>[2x]MGHHHHHHHHHHSSGHIEGRHMMAERKGTAKVDFLKKIEKEIQQKWDTERVFEVNASNLEKQTSKGKYFVTFPYPYMNGRLHLGHTFSLSKCEFAVGYQRLKGKCCLFPFGLHCTGMPIKACADKLKREIELYGCPPDFPDEEEEEEETSVKTEDIIIKDKAKGKKSKAAAKAGSSKYQWGIMKSLGLSDEEIVKFSEAEHWLDYFPPLAIQDLKRMGLKVDWRRSFITTDVNPYYDSFVRWQFLTLRERNKIKFGKRYTIYSPKDGQPCMDHDRQTGEGVGPQEYTLLKLKVLEPYPSKLSGLKGKNIFLVAATLRPETMFGQTNCWVRPDMKYIGFETVNGDIFICTQKAARNMSYQGFTKDNGVVPVVKELMGEEILGASLSAPLTSYKVIYVLPMLTIKEDKGTGVVTSVPSDSPDDIAALRDLKKKQALRAKYGIRDDMVLPFEPVPVIEIPGFGNLSAVTICDELKIQSQNDREKLAEAKEKIYLKGFYEGIMLVDGFKGQKVQDVKKTIQKKMIDAGDALIYMEPEKQVMSRSSDECVVALCDQWYLDYGEENWKKQTSQCLKNLETFCEETRRNFEATLGWLQEHACSRTYGLGTHLPWDEQWLIESLSDSTIYMAFYTVAHLLQGGNLHGQAESPLGIRPQQMTKEVWDYVFFKEAPFPKTQIAKEKLDQLKQEFEFWYPVDLRVSGKDLVPNHLSYYLYNHVAMWPEQSDKWPTAVRANGHLLLNSEKMSKSTGNFLTLTQAIDKFSADGMRLALADAGDTVEDANFVEAMADAGILRLYTWVEWVKEMVANWDSLRSGPASTFNDRVFASELNAGIIKTDQNYEKMMFKEALKTGFFEFQAAKDKYRELAVEGMHRELVFRFIEVQTLLLAPFCPHLCEHIWTLLGKPDSIMNASWPVAGPVNEVLIHSSQYLMEVTHDLRLRLKNYMMPAKGKKTDKQPLQKPSHCTIYVAKNYPPWQHTTLSVLRKHFEANNGKLPDNKVIASELGSMPELKKYMKKVMPFVAMIKENLEKMGPRILDLQLEFDEKAVLMENIVYLTNSLELEHIEVKFASEAEDKIREDCCPGKPLNVFRIEPGVSVS

Leucyl-tRNA synthetase (LRS), a class I AaRS, is particularly large and complex. Structurally, LRS contains an aminoacylation domain, a tRNA binding domain, and an editing domain, known as connective peptide 1 (CP1). HcLRS functions as the intracellular leucine sensor to modulate the activity of the mTOR complex 1 (mTORC1) by directly binding with RagD GTPase, the mediator of the AAs-dependent mTORC1 pathway. After screening truncations with different lengths, we found that deletion of the last 106 residues (N1071-1176C), designated as hcLRS_d106, gives improved crystals that diffract up to 2.5 Å resolution.

The asymmetric unit contains two non-crystallographically related hcLRS molecules with differences in B-factors and subtle differences in orientation of some of the peripheral domains. Luckily, in the current structure, the VC domain is visible even though there is no tRNA bound due to crystal contacts. LeuAMS, a stable analog of LeuAMP, was bound in the aminoacylation active site in our structure. Leucine, instead binds to a deep and narrow pocket formed by residues Tyr52, Tyr54, Leu594 and Ser597. Interestingly, residue His251 from the CP core is within 4 Å of the leucine, and the N atom from the imidazole ring of His251 is only 2.6 Å from the—OH group of Tyr54 suggesting a role of His251 in leucine binding. In our structure, a post-transfer editing analog Nva2AA (2′-(L-norvalyl) amino-2′-deoxyadenosine) is clearly bound at the editing active pocket. The residues involved in interaction with Nva2AA are mainly from the conserved ‘threonine-rich region’ (T-rich region) and the ‘GTG loop’ with one exception, Lys464, which is from a helix of I4ae insertion. Experimentally, the role of the tRNA-A76 3′-OH group in the mechanism of LRS deacylation was tested in E. coli LRS by replaced the terminal adenosine of tRNALeu with 3′-deoxyadenosine, the results showed that the 3′-OH group of A76 has a prominent role in deacylation reaction. Interestingly, a very well ordered water molecule which hydrogen-bonds to the 3′-OH group of tRNA-A76 is observed in our structure (W1 in Figure 3B and C).>MWIGVISLFPEMFKAITEFGVTGRAVKHNLLKVECWNPRDFTFDKHKTVDDRPYGGGPGMLMMVQPLRDAIHTAKAAAGEGAKVIYLSPQGRKLDQGGVTELAQNQKLILVCGRYEGIDERLIQTEIDEEWSIGDYVLTGGELPAMTLIDAVARFIPGVLGKQASAEEDSFADGLLDCPHYTRPEVLEGLTVPPVLMSGHHEEIRKWRLKQSLQRTWLRRPELLEGLALTDEQRKLLKEAQAEH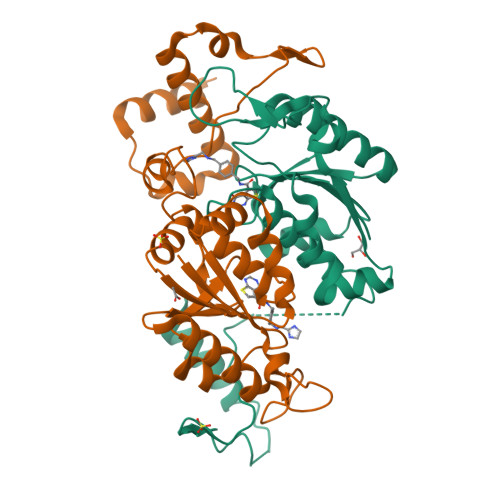NS[2x]8-(2-ethenyl-6-ethyl-4-methylphenyl)tetrahydro-7H-pyrazolo[1,2-d][1,4,5]oxadiazepine-7,9(8H)-dione 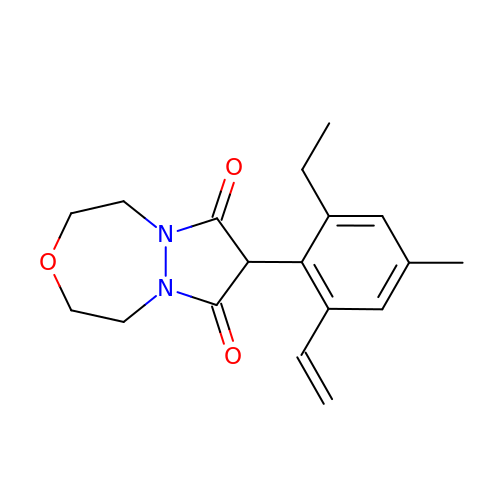| C18 H22 N2 O3 | CYYDMVKNZPACLF-UHFFFAOYSA-N>[2x]GSNRTLIVTTILEEPYVMYRKSDKPLYGNDRFEGYCLDLLKELSNILGFLYDVKLVPDGKYGAQNDKGEWNGMVKELIDHRADLAVAPLTITYVREKVIDFSKPFMTLGISILYRKGTPI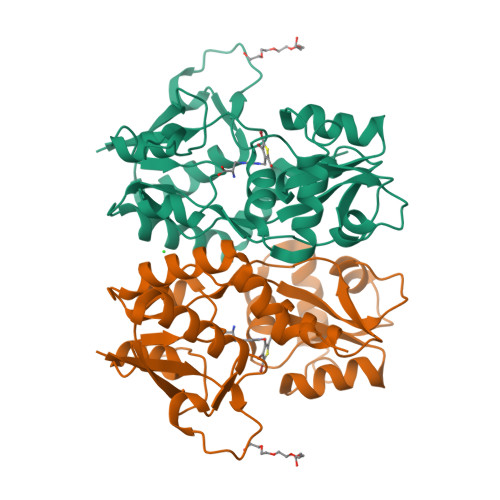DSADDLAKQTKIEYGAVRDGSTMTFFKKSKISTYEKMWAFMSSRQQSALVKNSDEGIQRVLTTDYALLMESTSIEYVTQRNCNLTQIGGLIDSKGYGVGTPIGSPYRDKITIAILQLQEEGKLHMMKEKWWRGNGCPS>[2x]AAGTQGAEFPELCSYTWEAVDTKNNMLYKINICGNMGVAQCGPSSAVCMHDL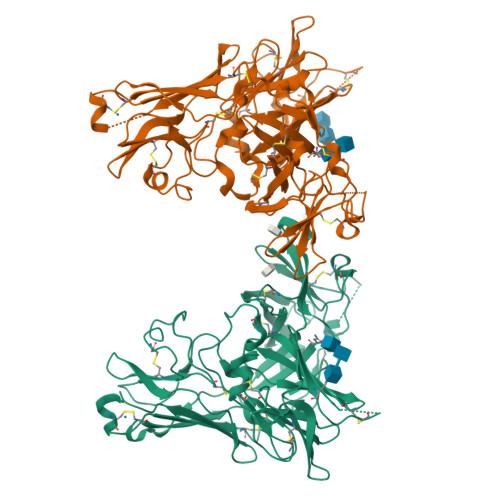KTDSFHSVGDSLLKTASRSLLEFNTTVNCKQQNHKIQSSITFLCGKTLGTPEFVTATDCVHYFEWRTTAACKKNIFKANKEVPCYAFDRELKKHDLNPLIKTSGAYLVDDSDPDTSLFINVCRDIEVLRASSPQVRVCPTGAAACLVRGDRAFDVGRPQEGLKLVSNDRLVLSYVKEGAGQPDFCDGHSPAVTITFVCPSERREGTIPKLTAKSNCRFEIEWVTEYACHRDYLESRSCSLSSAQHDVAVDLQPLSRVEASDSLFYTSEADEYTYYLSICGGSQAPICNKKDAAVCQVKKADSTQVKVAGRPQNLTLRYSDGDLTLIYFGGEECSSGFQRMSVINFECNQTAGNNGRGAPVFTGEVDCTYFFTWDTKYACV>[2x]GMEFLMKISHLDHLVLTVADIPTTTKFYEKVLGMKAVSFGSGRIALEFGHQKINLHQLGHEFEPKAQNVRTGSADLCFITDIDLSDAMEYVENQGVVIMEGPVKRTGAQG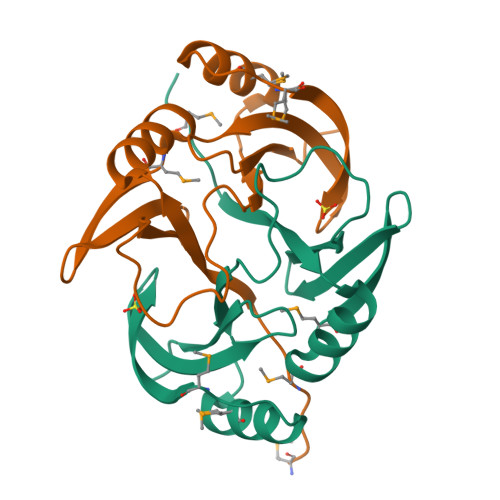AITSFYFRDPDGNLIEVSTYSNT> GSAREN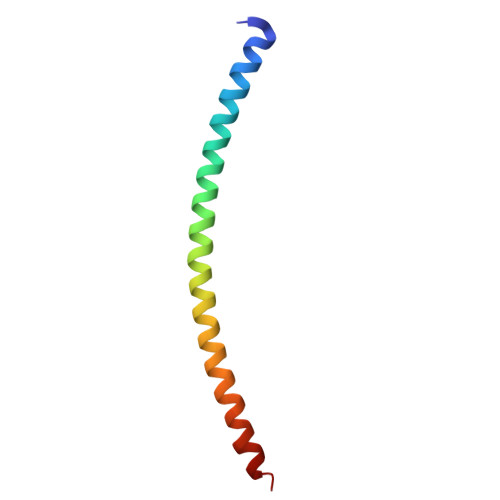EMDENLEQVSGIIGNLRHMALDMGNEIDTQNRQIDRIMEKADSNKTRIDEANQRATKMLW> MDSKQQCVKLNDGHFMPVLGFGTYAPPEVPRSKALEVTKLAIEAGFRHIDSAHLYNNEEQVGLAIRSKIADGSVKREDIFYTSKLWSTFHRPELVRPALENSLKKAQLDYVDLYLIHSPMSLKPGEELSPTDENGKVIFDIVDLCTTWEAMEKCKDAGLAKSIGVSNFNRRQLEMILNKPGLKYKPVCNQVECHPYFNRSKLLDFCKSKDIVLVAYSALGSQRDKRWVDPNSPVLLEDPVLCALAKKHKRTPALIALR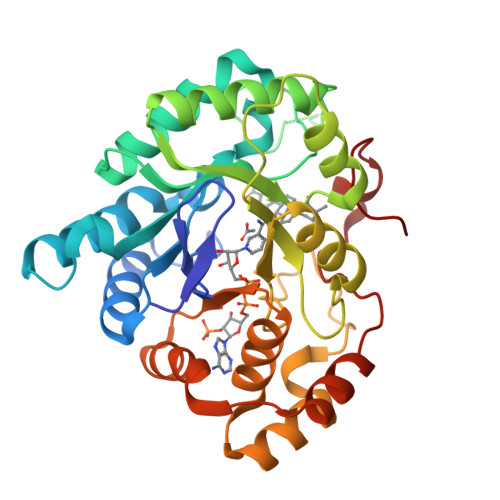YQLQRGVVVLAKSYNEQRIRQNVQVFEFQLTAEDMKAIDGLDRNLHYFNSDSFASHPNYPYSDEY> MGKTFPDVPADHWGIDSINYLVEKGAVKGNDKGMFEPGKELTRAEAATMMAQILNLPIDKDAKPSFADSQGQWYTPFIAAVEKAGVIKGTGNGFEPNGKIDRVSMASLLVEAY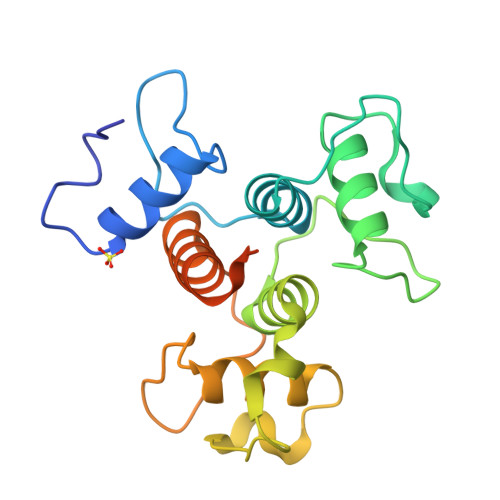KLDTKVNGTPATKFKDLETLNWGKEKANILVELGISVGTGDQWEPKKTVTKAEAAQFIAKTDKQFGTELEDPAANKARKEAELAAATAEN> CIPKWN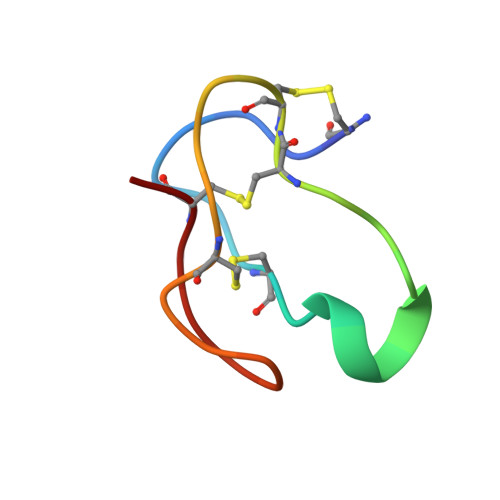RCGPKMDGVPCCEPYTCTSDYYGNCS> MTTIRGDDLSNQITQISGSSSKKEEEKKKQQMLTGVLGLQPTMANHPVLGVFLPKYAKQNGGNVDKTAFRLDLIRMLALHRLNTKT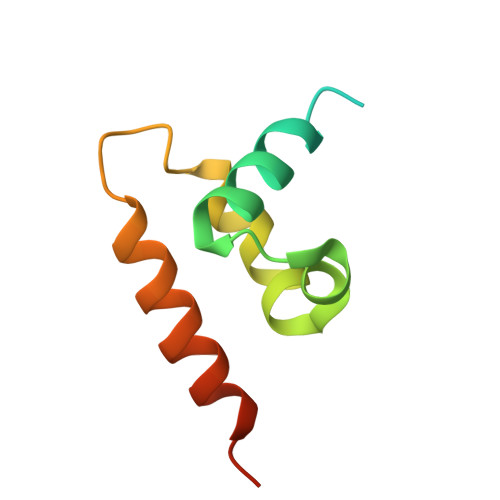GSD> MSISISYSTTYSGWTVADYLADWSAYFGDVNHRPGQVVDGSNTGGFNPGPFDGSQYALKSTASDAAFIAGGDLHHTLFSNPSHTLWGKLDSIALGDTLTGGASSGGYALDSQEVSFSNLGLDSPIAQGRDGTVHKVVYGLMSGDSSALQGQIDAL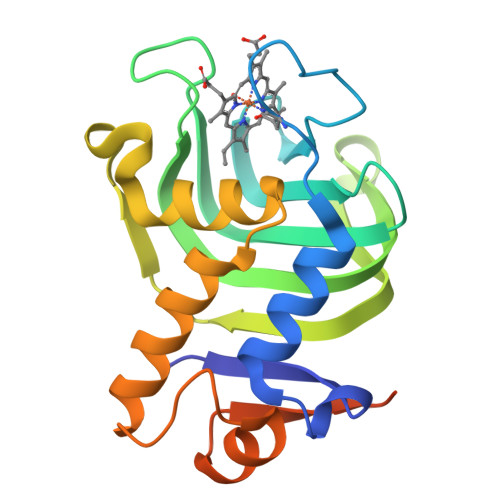LKAVDPSLSINSTFDQLAAAGVAHATPAAAAAEVGVVGVQELPHDLALAA>GPLGSKQARKDMALQHAVDLLEKMLADEEKKLTEFNLGDPLFESANDDPIKTLEEIIQEGDDVVGAHQLVVTQIKLRVQRNRRLADEIIREQLTDIRKVFSDKFEKLEQGIQNSYLLLDKLKTPFQDMRCLFEVANEQFNDTPVPPQYKEKFMVCLKQIVQYAVNSSSKLEKFVMLKIKTKKDDIKDRVTYTCMKYLLMAMQGTGGPKAINNEEHAKLFFKQLSNYDDLTDANHDGLELIKKLDKEQK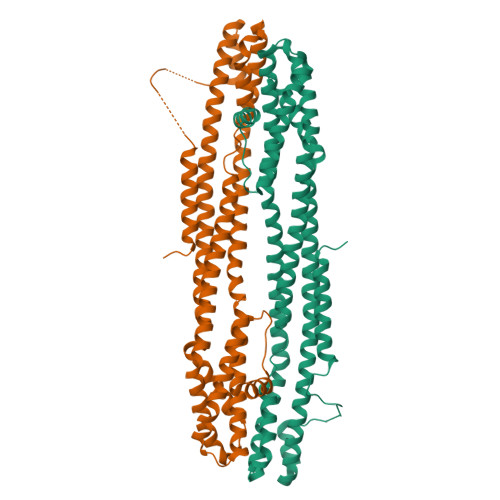EVAFHVNNFTHLVTTLGMALYKEGHQKNDEAMLGMHTPITMLSDQVRVLILYLIDEIVHAIHTNSNQSNDELIDGLKPKVRIVINEFHATLMMGIDKMKFYSLNELREIVNDKINED[4x]N-[3,4-dioxo-2-(4-{[4-(trifluoromethyl)benzyl]amino}piperidin-1-yl)cyclobut-1-en-1-yl]-3,5-dimethyl-1,2-oxazole-4-sulfonamide | C22 H23 F3 N4 O5 S | 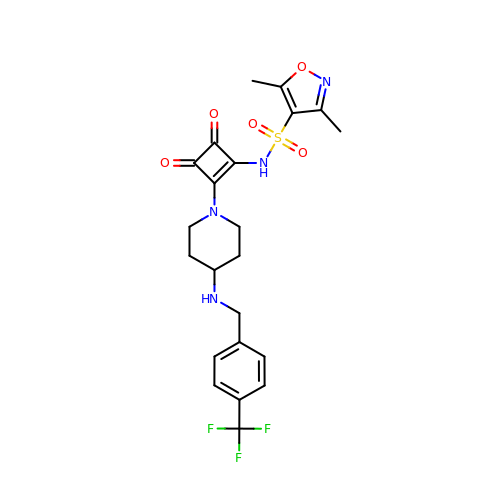WFHJESWCVOQIPR-UHFFFAOYSA-N>[2x]SSPVAQKYDYILVGGGTAACVLANRLSADGSKRVLVLEAGPDNTSRDVKIPAAITRLFRSPLDWNLFSELQEQLAERQIYMARGRLLGGSSATNATLYHRGAAGDYDAWGVEGWSSEDVLSWFVQAETNADFGPGAYHGSGGPMRVENPRYTNKQLHTAFFKAAEEVGLTPNSDFNDWSHDHAGYGTFQVMQDKGTRADMYRQYLKPVLGRRNLQVLTGAAVTKVNIDQAAGKAQALGVEFSTDGPTGERLSAELAPGGEVIMCAGAVHTPFLLKHSGVGPSAELKEFGIPVVSNLAGVGQNLQDQPACLTAAPVKEKYDGIAISDHIYNEKGQIRKRAIASYLLGGRGGLTSTGCDRGAFVRTAGQALPDLQVRFVPGMALDPDGVSTYVRFAKFQSQGLKWPSGITMQLIACRPQSTGSVGLKSADPFAPPKLSPGYLTDKDGADLATLRKGIHWARDVARSSALSEYLDGELFPGSGVVSDDQIDEYIRRSIHSSNAITGTCKMGNAGDSSSVVDNQLRVHGVEGLRVVDASVVPKIPGGQTGAPVVMIAERAAALLTGKATIGASAAAPATVAA

Fatty-acid photodecarboxylase (FAP), together with protochlorophyllide oxidoreductase and DNA photolyases, is a member of the rare class of photoenzymes that require light to initiate each catalytic event. Absorption of a blue-light photon by the flavin adenine dinucleotide (FAD) cofactor within FAP triggers the decarboxylation of the fatty-acid substrate, which leads to the formation of a hydrocarbon molecule and CO2. The recently published high-resolution (1.8 Å) structure of FAP, determined from cryo-crystallo­graphic synchrotron data combined with UV–Vis absorbance spectra, revealed a bent oxidized FAD in the dark state. Forward electron transfer from the fatty-acid substrate to the photoexcited FAD occurs in 300 ps and is accompanied by concomitant decarboxylation of the latter, as shown by time-resolved visible and infrared (IR) absorption spectroscopies, respectively.

Here, we extend the study of Sorigué et al. by carrying out the refinement of intermediate-state structures against extrapolated structure factors at 20 ps, 900 ps, 300 ns and 2 µs. We present additional TR-SFX data collected at a pump–probe delay of 900 ps at three different pump-laser power densities that explain why the particular pump-laser power density was chosen for the TR-SFX experiment reported by Sorigué et al.. In order to model the structural changes that had occurred at the different time points, structure-factor extrapolation was carried out using Xtrapol8, which estimates the structure-factor amplitudes F ext that would have been measured for each pump–probe data set if the photo-triggered intermediate were present in the crystals at 100% occupancy (equation 1). The occupancy of intermediate states was determined to be between 25% and 35% for the four time delays. Three possible explanations can be offered: (i) the spatial overlap between the pump and probe laser changed slightly, (ii) the apparent difference reflects the noise level of the data or (iii) at 900 ps a positive peak due to photodecarboxylated CO2 compensates part of the negative peak on the carboxyl group.> MDTEVYESPYADPEEIRPKEVYLDRKLLTLEDKELGSGNFGTVKKGYYQMKKVVKTVAVKILKNEANDPALKDELLAEANVMQQLDNPYIVRMIGICEAESWMLVMEMAELGPLNKYLQQNRHVKDKNIIELVHQ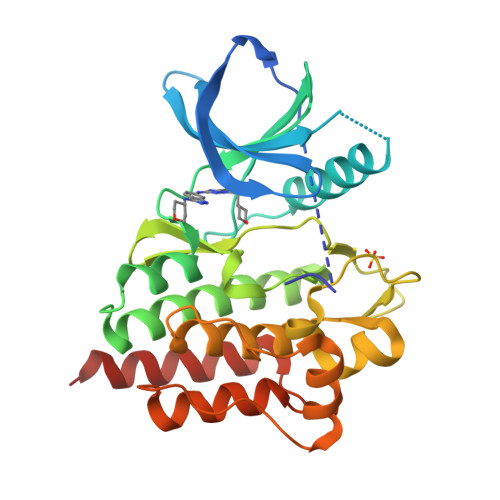VSMGMKYLEESNFVHRDLAARNVLLVTQHYAKISDFGLSKALRADENYYKAQTHGKWPVKWYAPECINYYKFSSKSDVWSFGVLMWEAFSYGQKPYRGMKGSEVTAMLEKGERMGCPAGCPREMYDLMNLCWTYDVENRPGFAAVELRLRNYYYDVVNHHHHHH> RPQGATVSLWETVQKWREYRRQCQRSLTEDPPPATDLFCNRTFDEYACWPDGEPGSFVNVSCPWYLPWASSVPQGHVYRFCTAEGLWLQKDNSSLPWRDLSECEESKRGERSSPEEQLLFLYYIYTVGYALSFSALVIASAILLGFRHLHCTRNYIHLNLFASFILRALSVFIKDAALKWMYSTRAQQHEWDGLLRYQDSLSCRLVFLLMQYCVAANYYWLLVEGVYLYTLLAFSVASEQWIFRLYVSIGWGVPLLFVVPWGIVKYLAEDEGCWTRNSNMNYWLIIRLPILFAIGVNFLIFVRVICIVVSKLKANEMCKTDIQCRLAKSTLTLIPLLGTHEVIFAFVMDEHARGTLRFIKLFTELSFTSFQGLMVAILYCFV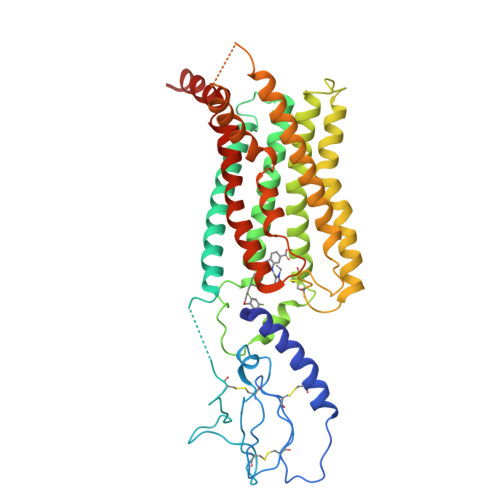NNEVQLEFRKSWERWRL> MQRNTYNKVGLYILSLAMLFVFIIILTAKIPFCFTSDCSFIGLKKLVLTNIVPIVCFVFFLFSIYFYNRLKNITKYNGQDSVKITSCQSESYESLTFLATYIVPFMGFSFEDMQKNIAYLLLVVVIGIIFIKTDKYYANPTLALFGFKLYRVNILHPGSGETKNLIAISNDVLKVD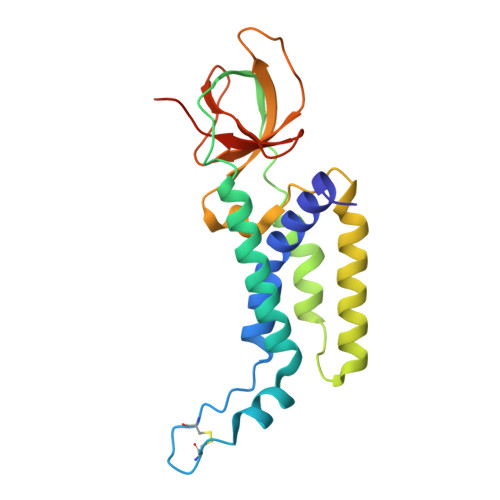DNVYYSFFDEFVFIARKKIDYKDDDDK>[8x]MTTTSPLHFVTLLGSLRKASFNAAVARALPEIAPEGIAITPLGSIGTFPHYSQDVQEEGFPAPVLTMAQQIATADAVVIVTPEYNYSVPGVLKNAIDWLSRVSPQPLA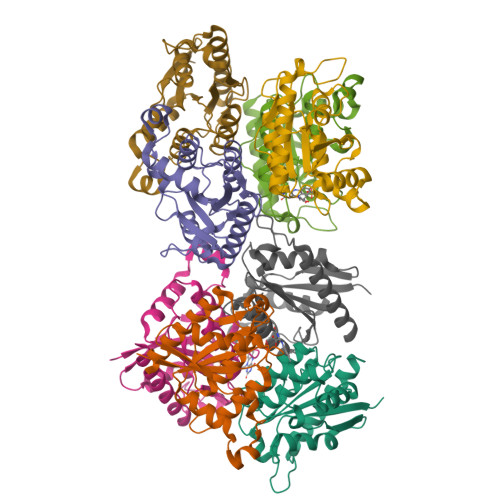GKPVALVTASPGMIGGARAQNHLRQSLVFLDAYVLNRPEAMIGQVTGKVDAQTLELSDVATREFLARQLDALAALARTLSPRAITHHHHHH> MNKDQAEKYQERSLRQKYNLLHVLPTLNSRALSGLYYKNFHNSVKRYQIMLPEQLKSGKFCSHCGCVYVPNFNASLQLT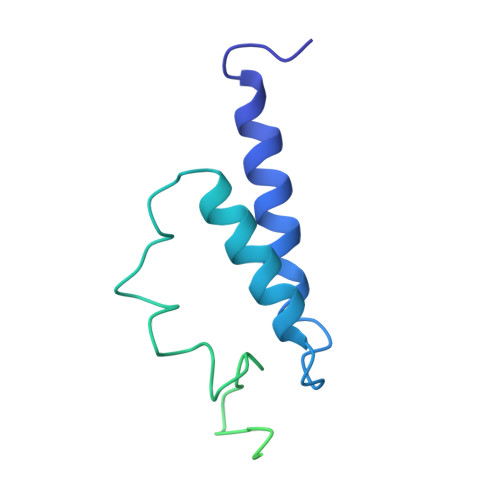TNTEQGDSDELGGESMEGPKKCIQVNCLNCEKSKLFEWKSEFVVPTFGQDVSPMINSTSSGKVSYAVKKPQKSKTSTGKERSKKRKLNSLTNLLSKRNQEKKMEKKKSSSLSLESFMKS> MIIPALNLIDGTVVRLHQGDYARQRDYGNDPLPRLQDYAAQGAGVLHLVDLTGAKDPAKRQIPLIKTLVAGVNVPVQVGGGVRTEEDVAALLKAGVARVVIGSTAVKSPDVVKGWFERFGAQALVLALD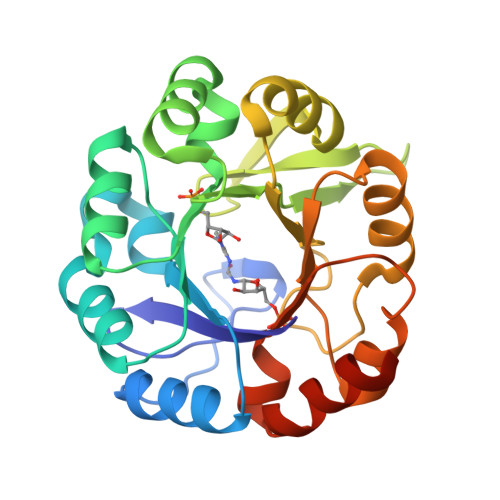VRIDEHGTKQVAVSGWQENSGVSLEQLVETYLPVGLKHVLCTDISRAGTLAGSNVSLYEEVCARYPQIAFQSSGGIGDIDDIAALRGTGVRGVIVGRALLEGKFTVKEAIQCWQNVKGHHHHHH> MTLRAAVFDLDGVLALPAVFGVLGRTEEALALPRGLLNDAFQKGGPEGATTRLMKGEITLSQWIPLMEENCRKCSETAKVCLPKNFSIKEIFDKAISARKINRPMLQAALMLRKKGFTTAILTNTWLDDRAERDGLAQLMCELKMHFDFLIESCQVGMVKPEPQIYKFLLDTLKASPSEVVFLDDIGANLKPARDLGMVTILVQDTDTALKELEKVTGIQLLNTPAPLPTSCNPSDMSHGYVTVKPRVRLHFVELGSGPAVCLCHGFPESWYSWRYQIPALAQAGYRVLAMDMKGYGESSAPPEIEEYCME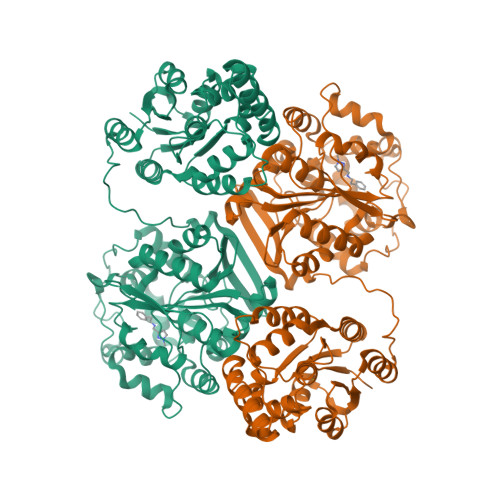VLCKEMVTFLDKLGLSQAVFIGHDWGGMLVWYMALFYPERVRAVASLNTPFIPANPNMSPLESIKANPVFDYQLYFQEPGVAEAELEQNLSRTFKSLFRASDESVLSMHKVCEAGGLFVNSPEEPSLSRMVTEEEIQFYVQQFKKSGFRGPLNWYRNMERNWKWACKSLGRKILIPALMVTAEKDFVLVPQMSQHMEDWIPHLKRGHIEDCGHWTQMDKPTEVNQILIKWLDSDARNPPVVSKMHHHHHH> SALLNTSGLPAVLEPFSRTPVIPVASPDPALVNNPVVAATEPSVVKIRSLAPRCQKVLEGTGFVISPDRVMTNAHVVAGSNNVTVYAGDKPFEATVVSYDPSVDVAILAVPHLPPPPLVFAAEPAKTGADVVVLGYPGGGNFTATPARIREAIRLSGPDIYGDPEPVTRDVYTIRADVEQGDSGGPLIDLNG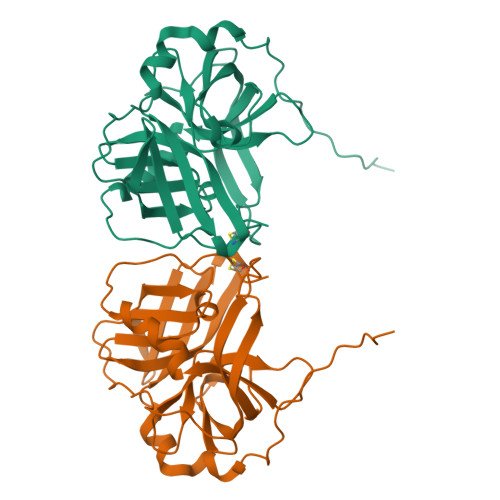QVLGVVFGAAIDDAETGFVLTAGEVAGQLAKIGATQPVGTGACVS>MSDQPIIRRRQVKTGISDARANNAKTQSQYQPYKDAAWGFINHWYPALFTHELEEDQVQGIQICGVPIVLRRVNGKVFALKDQCLHRGVRLSEKPTCFTKSTISCWYHGFTFDLETGKLVTIVANPEDKLIGTTGVTTYPVHEVNGMIFVFVREDDFPDEDVPPLAHDLPFRFPERSEQFPHPLWPSSPSVLDDNAVVHGMHRTGFGNWRIACENGFDNAHILVHKDNTIVHAMDWVLPLGLLPTSDDCIAVVEDDDGPKGMMQWLFTDKWAPVLENQELGLKVEGLKGRHYRT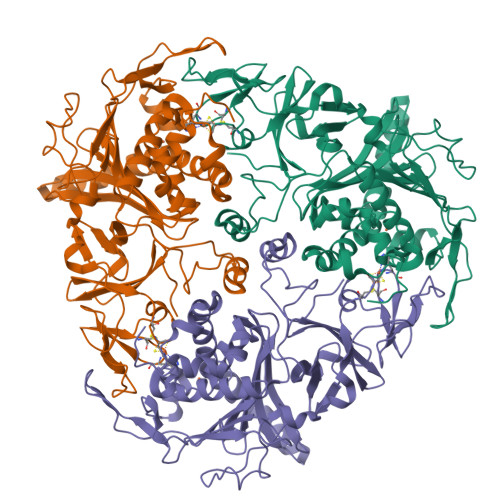SVVLPGVLMVENWPEEHVVQYEWYVPITDDTHEYWEILVRVCPTDEDRKKFQYRYDHMYKPLCLHGFNDSDLYAREAMQNFYYDGTGWDDEQLVATDISPITWRKLASRWNRGIAKPGRGVAGAVKDTSLIFKQTADGKRPGYKVEQIKEDH[6x]>[4x]MDSYQTPLSSRYASKEMSKLFSSGARFGTWRKLWLNLAIAEKELGLAISDAAIEQMKANLELDEAQMKVAAEEEKKRRHDVMAHVHTFGTVAPEAAGIIHLGATSCYVTDNADLIFLRDGLDILLPKLATVISRLANFAKQYRDLPTLGFTHFQPAQLTTVGKRATLWIQELLWDLRNLQRARDDLGFRGVKGTTGTQA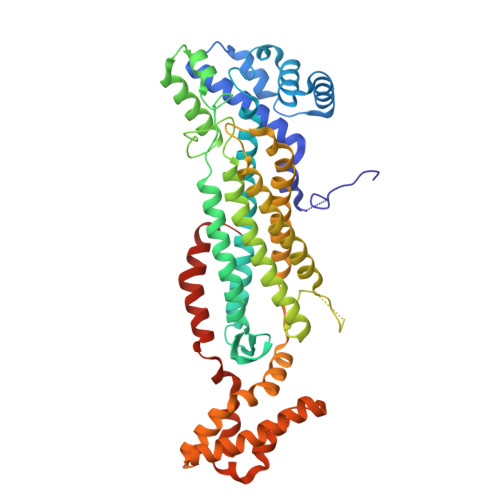SFLALFDGDHAKVEALDKRVTELFGFPYAYPVTGQTYSRKIDADVLGPLSSFGATVHKIATDIRLLANLKEIEEPFEKDQIGSSAMAYKRNPMRCERACSLARHLMAIYQNTLMTSSVQWLERTLDDSANRRVTIPEAFLTADILLTTLQNISEGLVVYPRVIGRRISQELPFMATENIIMAIVKAGGDRQECHEKIRVLSHQAGAVVKEEGGENDLIDRVKNDEYFKPIWGQLDALLDPRTFVGRAPEQVDGFLKEWVEPALKPYEEALKNVKTAELSV> GLGGGLVEIPRAPDIDPLEALMTNPVVPESKRFCWNCGRPVGRSDSETKGASEGWCPYCGSP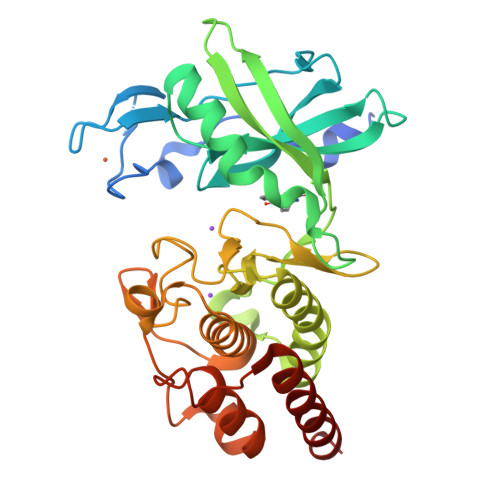YSFLPQLNPGDIVAGQYEVKGCIAHGGLGWIYLALDRNVNGRPVVLKGLVHSGDAEAQAMAMAERQFLAEVVHPSIVQIFNFVEHTDRHGDPVGYIVMEYVGGQSLKRSKGQKLPVAEAIAYLLEILPALSYLHSIGLVYNDLKPENIMLTEEQLKLIDLGAVSRINSFGYLYGTPGFQAPEIVRTGPTVATDIYTVGRTLAALTLDLPTRNGRYVDGLPEDDPVLKTYDSYGRLLRRAIDPDPRQRFTTAEEMSAQLTGVLREVVAQDTG>MASFEGARLSMRSRRNGTMGSTRTLYSSVSRSTDVSYSDSDLVNFIQANFKKRECVFFTRDSKAMENICKCGYAQSQHIEGTQINQNEKWNYKKHTKEFPTDAFGDIQFETLGKKGKYLRLSCDTDSETLYELLTQHWHLKTPNLVISVTGGAKNFALKPRMRKIFSRLIYIAQSKGAWILTGGTHYGLMKYIGEVVRDNTISRNSEENIVAIGIAAWGMVSNRDTLIRSCDDEGHFSAQYIMDDFTRDPLYILDNNHTHLLLVDNGCHGHPTVEAKLRNQLEKYISERTSQDSNYGGKIPIVCFAQGGGRETLKAINTSVKSKIPCVVVEGSGQIA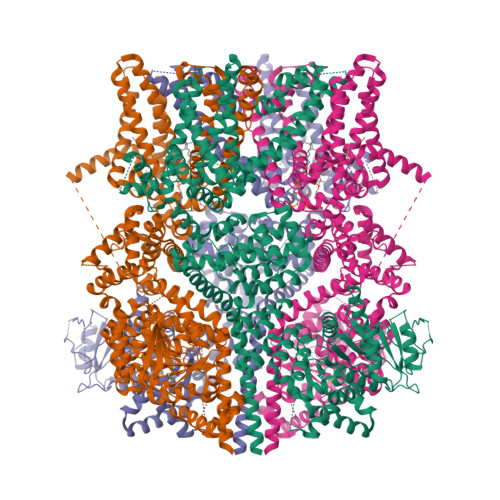DVIASLVEVEDVLTSSMVKEKLVRFLPRTVSRLPEEEIESWIKWLKEILESSHLLTVIKMEEAGDEIVSNAISYALYKAFSTNEQDKDNWNGQLKLLLEWNQLDLASDEIFTNDRRWESADLQEVMFTALIKDRPKFVRLFLENGLNLQKFLTNEVLTELFSTHFSTLVYRNLQIAKNSYNDALLTFVWKLVANFRRSFWKEDRSSREDLDVELHDASLTTRHPLQALFIWAILQNKKELSKVIWEQTKGCTLAALGASKLLKTLAKVKNDINAAGESEELANEYETRAVELFTECYSNDEDLAEQLLVYSCEAWGGSNCLELAVEATDQHFIAQPGVQNFLSKQWYGEISRDTKNWKIILCLFIIPLVGCGLVSFRKKPIDKHKKLLWYYVAFFTSPFVVFSWNVVFYIAFLLLFAYVLLMDFHSVPHTPELILYALVFVLFCDEVRQWYMNGVNYFTDLWNVMDTLGLFYFIAGIVFRLHSSNKSSLYSGRVIFCLDYIIFTLRLIHIFTVSRNLGPKIIMLQRMLIDVFFFLFLFAVWMVAFGVARQGILRQNEQRWRWIFRSVIYEPYLAMFGQVPSDVDSTTYDFSHCTFSGNESKPLCVELDEHNLPRFPEWITIPLVCIYMLSTNILLVNLLVAMFGYTVGIVQENNDQVWKFQRYFLVQEYCNRLNIPFPFVVFAYFYMVVKKCFKCCCKEKNMESNACCFRNEDNETLAWEGVMKENYLVKINTKANDNSEEMRHRFRQLDSKLNDLKSLLKEIANNIKSNSLEVLFQGPDYKDDDDKAHHHHHHHHHH[4x]> MGESLDRCIDDINRAVDSMS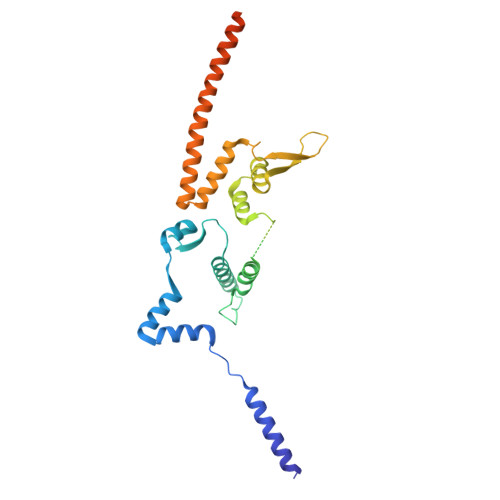TLYFKPPGIFHNAILQGASNKASIRKDITRLIKDCNHDEAYLLFKVNPEKQSVSRRDGKEGVFDYVIKRDTDMKRNRRLGRPGEKPIIHVPKEVYLNKDRLDLNNKRRRTATTSGGGLNGFIFDTDLIGSSVISNSSSGTFKALSAVFKDDPQIQRLLYALENGSVLMEEESNNQRRKTIFVEDFPTDLILKVMAEVTDLWPLTEFKQDYDQLYHNYEQLSSKLRFIKKEVLLQDDRLKTMSQYHPSSSHDVAKIIRKEKDEIRRLEMEIANLQE>MSAKKIVLKSSDGESFEVEEAVALESQTIAHMVEDDCVDNGVPLPNVTSKILAKVIEYCKRHVEAAASKAEAVEGAATSDDDLKAWDADFMKIDQATLFELILAANYLNIKNLLDLTCQTVADMIKGKTPEEIRTTFNIKNDFTPEEEEEVRRENQWAFE[2x];>MAEEEEVEEGRSSSSAILDLPEPLLLHILSFLTDVRSRHRAALACGRMRAAERATRSELSLRGDPRSPGFLFLSHAFRFPALEHLDLSLVSPWGHPLLSSVPPCGGGGGGAPSASSSSGMNVYHPEAISEQNAFIAARLAGCFPAVTSLAVYCRDPTTLANLTPHWQASLRRVKLVRWHQRPPTLPDGADLEPLLETCAALRELDLSEFYCWTEDVVRALTTHPSATAALTHLDLGLAAATDGFKSSELGPIAASCPNLRKLVAPCLFNPRFSDCVGDDALLSLATSCPRLTVLRLSEPFEAAANIQREEAAITVAGLVAFFAALPALEDFTMDLQHNVLEAAPAMEALARRCPRIKFLTLGSFQGLCKASWLHLDGVAVCGGLESLYMKNCQDLTDASLAAIGRGCRRLAKFGIHGCDLVTSAGIRRLAFTLRPTLKEVTVLHCRLLHTAECLTALSPIRDRIESLEINCVWNTTENLYFQSLGSWEMLRSLSLWFSAGQLLSPLISAGLDSCPVLEEISIKVEGDCRTCPRPAPRTIFGLSDLAGFPVLAKMKLDLSEAVGYALTAPTGQMDLSLWERFYLHGIESLQTLYELDYWPPQDKDVHHRSLTLPA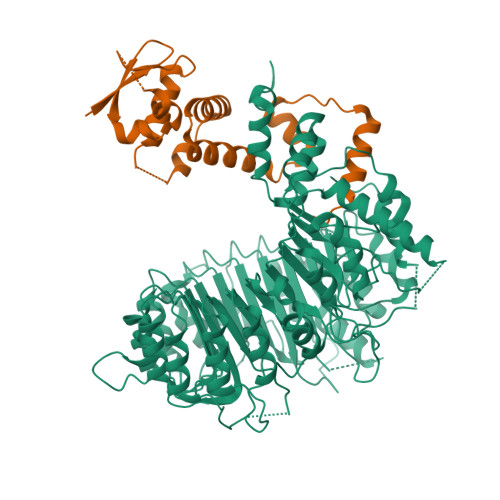VGLIQRCVGLRKLFIHGTTHEHFMTFFLSIPNLRDMQLREDYYPAPENDLMFTEMRAESWLRFEVQLNSRQIDD[2x]> GGCUUAUCAAGAGAGGGCGAGCGACUGGCGCGAAGACCCCCGGCA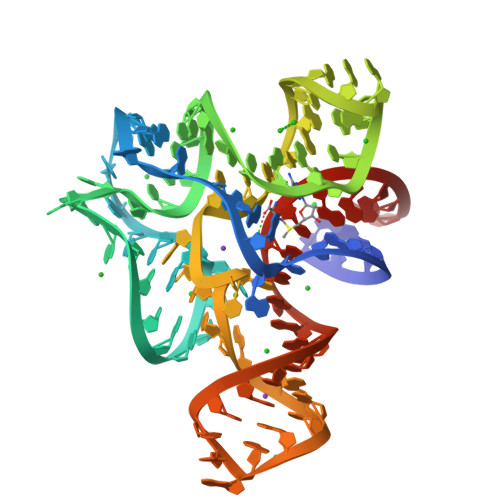ACCAGAAAUGGUGCCAAUUCCUGCAGCGGAAACGUUGAAAGAUGAGCCG> MTQEQANQSETKPAFDFKPFAPGYAEDPFPAIERLREATPIFYWDEGRSWVLTRYHDVSAVFRDERFAVSREEWESSAEYSSAIPELSDMKKYGLFGLPPEDHARVRKLVNPSFTSRAIDLLRAEIQRTVDQLLDARSGQEEFDVVRDYAEGIPMRAISALLKVPAECDEK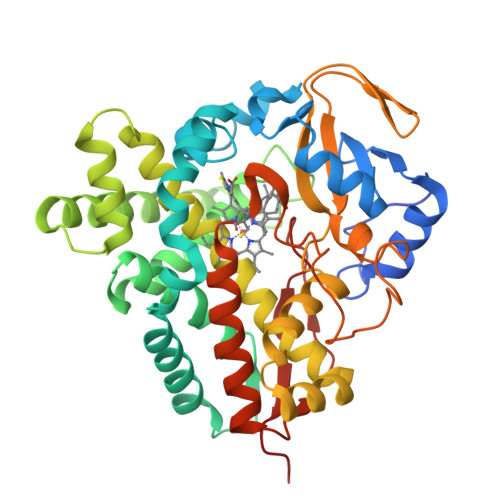FRRFGSATARALGVGLVPRVDEETKTLVASVTEGLALLHGVLDERRRNPLENDVLTMLLQAEADGSRLSTKELVALVGAIIAAGTDTTIYLIAFAVLNLLRSPEALELVKAEPGLMRNALDEVLRFENILRIGTVRFARQDLEYCGASIKKGEMVFLLIPSALRDGTVFSRPDVFDVRRDTSASLAYGRGPHVCPGVSLARLEAEIAVGTIFRRFPEMKLKETPVFGYHPAFRNIESLNVILKPSKAG>GSMAPAGVPENTSLENIPVIVSKCREAFNDDANRDLKKRKQVLRSLLNLVEENTDEFCKAIHRDRRRHRDETVVMEILPLRNEVWHLIEHMDEYVKPVKPTMEGAAALDDCELQYEPLGVVLVIGTWNYPLLLILQPLLGALAAGNTAVIKPSELAPATAELLTKLLPKYVSSDVVGIVNGGVSETTAVLKERFDHILYTGSARVAEIVMAAAAKHLTPVTLELGGKSPVVVDDTCADNMKVVAERIMWGKIINAGQTSIAPDYVVVEKSMESVLVDALAEARKAMLGDKFLKVLKGELLVKQKQQFLEESDYPRIVNASHFQRLMEFMKGGKVAVGGEADEATLTIAPTILTNIDPTHPVMQEEIFGPILPVLTYENEKDILKIINSREKPLALYVFSNNKRFIRGVESRTSSGAVVVNDVVVHAGADGLPFGGVGRSGMGAYHGRYSFETFSHRRPVMRRGFLFSSIDTVRFPPYTTAKSRVLNSLLKPSAEVAGAVGRSVWGVAALARVVEVGYHYMRFLMAGETTPAPSSSEPFSKSPRSNE[2x]

Part of the initial identifications suggested a specific SAR between the function conferred by an individual gene and aminomethylphenoxy derivatives, mediated by the methylamine moiety shared by the compounds. This gene encodes a protein, TbALDH3 that potentially functions as a trypanosomal FALDH based on our crystallographic and biochemical characterizations. The monomer structure comprises 485 residues from A6 to K490, and adopts a canonical ALDH fold that is composed of an N-terminal NAD-binding domain, a catalytic domain and an oligomerization domain embracing the second subunit of the dimer. Interestingly, this C-terminal structural element strikingly resembles the ‘gatekeeper helix’ that is unique to FALDHs and is involved in regulating enzyme activity and substrate specificity. Moreover, the difference in MS between M1 and M-A1 correlates well with the transition from aldehyde (-CHO) to carboxylic acid (-CO2H), as well as M2 and M-A2, suggesting it is highly likely that M1 and M2 are the aldehyde precursors of the carboxylic acids M-A1 and M-A2 respectively. These data collectively support the notion that MAOa-TbALDH3 can metabolize the aminomethylphenoxy derivatives in a stepwise manner, i.e. the methylamine group in the structure is first converted by MAOa into an aldehyde, and then is further metabolized into a carboxylic acid by TbALDH3.

To understand the reaction catalyzed by TbALDH3 at molecular level, we obtained crystals of the aldehyde-NAD-TbALDH3 complex. A micro-reaction chamber was designed to serve as a physical barrier between the two reactions as well as to minimize the reverse reaction; meanwhile, a cysteine to serine mutation (C259S) was introduced in TbALDH3 to entrap the hyperactive aldehyde metabolites by abolishing the nucleophilic attack on the carbonyl carbon of the aldehyde. The NAD cofactor is located in an extended pocket rendered by a Rossmann fold. There are two hydrogen bonds formed between E365 and the hydroxyl groups of the ribose of the nicotinamide, establishing the key interactions between NAD with TbALDH3 in addition to an H2O-bridge that connects the carboxylate group of the nicotinamide to Y444 and T200. In this structure, the benzaldehyde benzoxaborole substrate exhibits distinctive electron density, being nestled into the substrate funnel and adjacent to the nicotinamide. Specifically, in the catalytic pocket, its aldehyde group directly contacts the catalytic residue (C259S), and also connects to N128, a residue whose counterparts in other ALDHs are involved in the catalytic activity by directing the carbonyl carbon towards the nucleophilic carbon on the nicotinamide. Noticeably, the position of the substrate is relatively flexible as indicated by the B-factor.> HH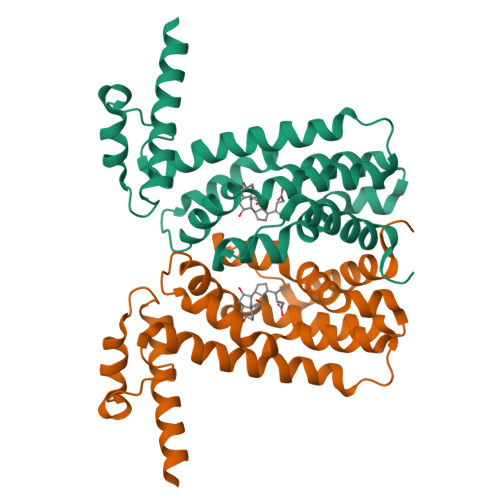HHHHMNSNMNSNRTPSQKVLARQEKIKAVALELFLTKGYQETSLSDIIKLSGGSYSNIYDGFKSKEGLFFEILDDICKKHFHLIYSKTQEIKNGTLKEILTSFGLAFIEIFNQPEAVAFGKIIYSQVYDKDRHLANWIENNQQNFSYNILMGFFKQQNNSYMKKNAEKLAVLFCTMLKEPYHHLNVLINAPLKNKKEQKEHVEFVVNVFLNGINSSKA>AMNNTIINSLIGGDDSIKRSNVFAVDSQIPTLYMPQYISLSGVMTNDGPDNQAIASFEIRDQYITALNHLVLSLELPEVKGMGRFGYVPYVGYKCINHVSISSCNGVIWEIEGEELYNNCINNTIALKHSGYSSELNDISIGLTPNDTIKEPSTVYVYIKTPFDVEDTFSSLKLSDSKITVTVTFNPVSDIVIRDSSFDFETFNKEFVYVPELSFIGYMVKNVQIKPSFIEKPRRVIGQINQPTATVTEVHAATSLSVYTKPYYGNTDNKFISYPGYSQDEKDYIDAYVSRLLDDLVIVSDGPPTGYPESAEIVEVPEDGIVSIQDADVYVKIDNVPDNMSVYLHTNLLMFGTRKNSFIYNISKKFSAITGTYSDATKRTIFAHISHSINIIDTSIPVSLWTSQRNVYNGDNRSAESKAKDLFINDPFIKGIDFKNKTDIISRLEVRFGNDVLYSENGPISRIYNELLTKSNNGTRTLTFNFTPKIFFRPTTITANVSRGKDKLSVR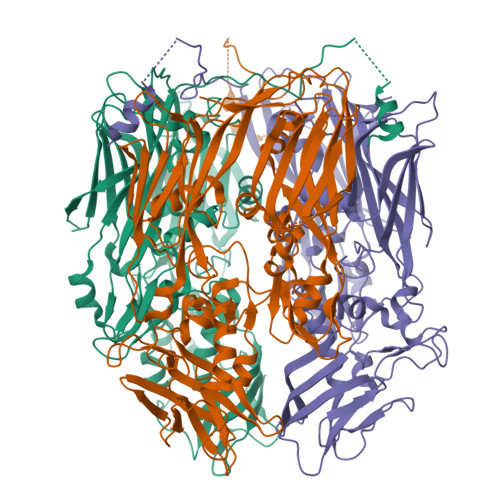VVYSTMDVNHPIYYVQKQLVVVCNDLYKVSYDQGVSITKIMG[3x]>[4x]AMRQCAIYGKGGIGKSTTTQNLVAALAEMGKKVMIVGCDPKADSTRLILHSKAQNTIMEMAAEAGTVEDLELEDVLKAGYGGVKCVESGGPEPGVGCAGRGVITAINFLEEEGAYEDDLDFVFYDVLGDVVCGGWAMPIRENKAQEIYIVCSGEMMAMYAANN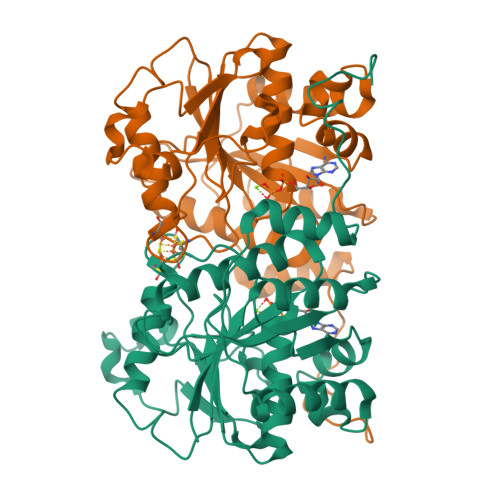ISKGIVKYANSGSVRLGGLICNSRNTDREDELIIALANKLGTQMIHFVPRDNVVQRAEIRRMTVIEYDPKAKQADEYRALARKVVDNKLLVIPNPITMDELEELLMEFGIMEVEDESIVGKTAEEV[(R)-{2-[hydroxy(methyl)amino]-2-oxoethoxy}(4-methoxyphenyl)methyl]phosphonic acid | C11 H16 N O7 P | 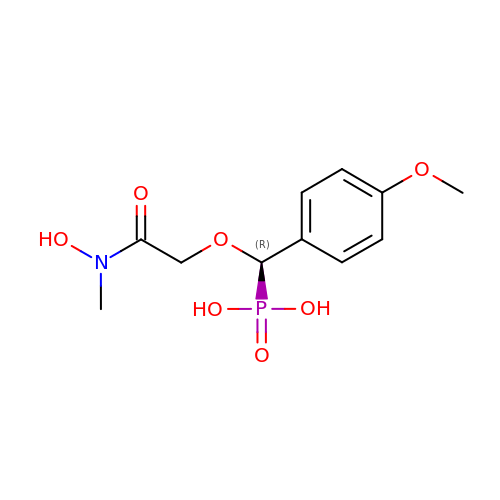LUULKKFHGAQKEF-LLVKDONJSA-N>PHFIVECSDNIREEADLPGLFAKVNPTLAATGIFPLAGIRSRVHWVDTWQMADGQHDYAFVHMTLKIGAGRSLESRQQAGEMLFELIKTHFAALMESRLLALSFEIEELHPTLNFK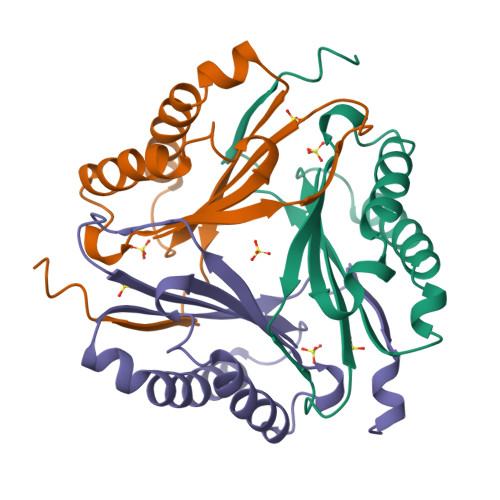QNNVHALFK[3x]> SHMPRWKRHI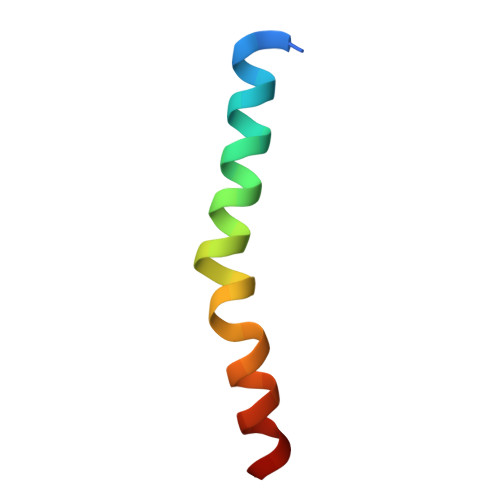SEQLRRRDRLQRQAFEEIILQYNKLL> MPFPVTTQGSQQTQPPQKHYGITSPISLAAPKETDCLLTQKLVETLKPFGVFEEEEELQRRILILGKLNNLVKEWIREISESKNLPQSVIENVGG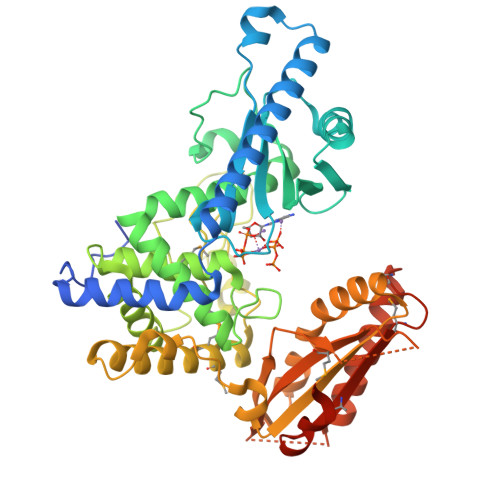KIFTFGSYRLGVHTKGADIDALCVAPRHVDRSDFFTSFYDKLKLQEEVKDLRAVEEAFVPVIKLCFDGIEIDILFARLALQTIPEDLDLRDDSLLKNLDIRCIRSLNGCRVTDEILHLVPNIDNFRLTLRAIKLWAKRHNIYSNILGFLGGVSWAMLVARTCQLYPNAIASTLVHKFFLVFSKWEWPNPVLLKQPEECNLNLPVWDPRVNPSDRYHLMPIITPAYPQQNSTYNVSVSTRMVMVEEFKQGLAITDEILLSKAEWSKLFEAPNFFQKYKHYIVLLASAPTEKQRLEWVGLVESKIRILVGSLEKNEFITLAHVNPQSFPAPKENPDKEEFRTMWVIGLVFKKTENSENLSVDLTYDIQSFTDTVYRQAINSKMFEVDMKIAAMHVKRKQLHQLLPSHVLQKKKKHSTEGV>[2x]MGSSHHHHHHSQDPNSSSARLQVDKLDYDIPTTENLYFQGSMRRSVYLDNTIEFLRGRVYLGAYDYTPEDTDELVFFTVEDAIFYNSFHLDFGPMNIGHLYRFAVIFHEI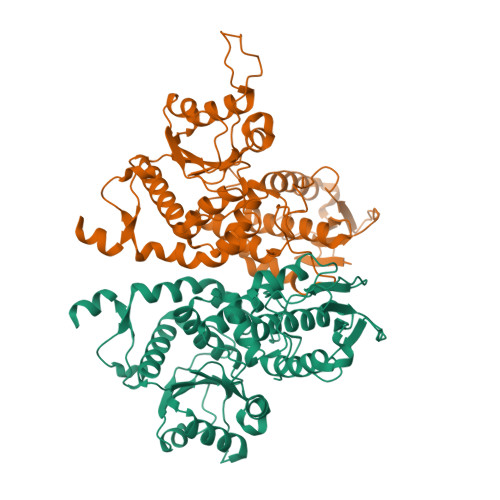LNDPENANKAVVFYSSASTRQRANAACMLCCYMILVQAWTPHQVLQPLAQVDPPFMPFRDAGYSNADFEITIQDVVYGVWRAKEKGLIDLHSFNLESYEKYEHVEFGDFNVLTPDFIAFASPQEDHPKGYLATKSSHLNQPFKSVLNFFANNNVQLVVRLNSHLYNKKHFEDIGIQHLDLIFEDGTCPDLSIVKNFVGAAETIIKRGGKIAVHCKAGLGRTGCLIGAHLIYTYGFTANECIGFLRFIRPGMVVGPQQHWLYLHQNDFREWKYTTRISLKPSEAIGGLYPLISLEEYRLQKKKLKD>[2x]MTVQMEYEKDVKVAALDGKKIAVIGYGSQGHAHAQNLRDSGRDVIIGVRPGKSFDKAKEDGFDTYTVAEATKLADVIMILAP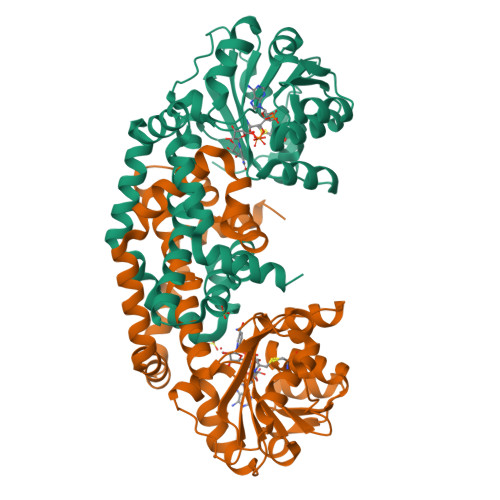DEIQQELYEAEIAPNLEAGNAVGFAHGFNIHFEFIKVPADVDVFMCAPKGPGHLVRRTYEEGFGVPALYAVYQDATGNAKNIAMDWCKGVGAARVGLLETTYKEETEEGLFGEQAVLCGGLTALIEAGFEVLTEAGYAPELAYFEVLHEMKLIVDLIYEGGFKKMRQSISNTAEYGDYVSGPRVITEQVKENMKAVLADIQNGKFANDFVNDYKAGRPKLTAYREQAANLEIEKVGAELRKAMPFVGKNDDDAFKIYN> GGTGGG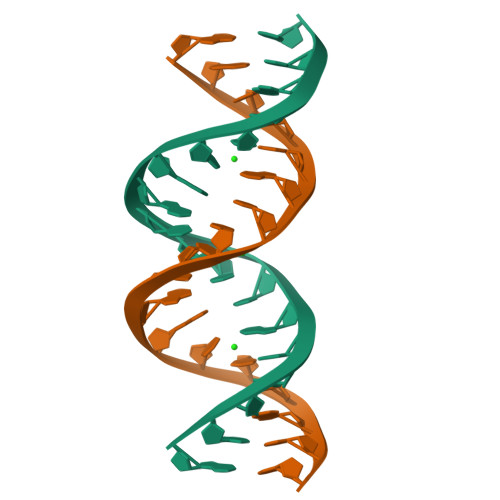TCTTGACCCACC>GAMEASEPVAETISKRFWTLIKMLRFYVVLRRFGYIDPLIYSIDPKQIKDVLSEALREFVSYTSSSSSRSIVIYDDPKNPVTAQAPCLVVAKRDEIPQNFPSIYRYTIYKIDKSSEYCISPLVVNDKYATLITPNESVIKEFFDKLDSNIQYARVLA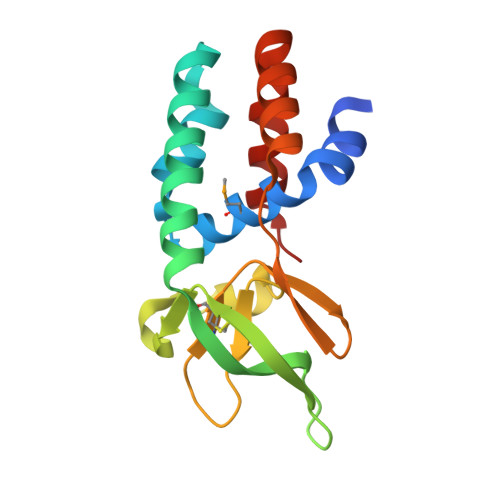SLAVGGE[9x]> MSLRPCFVSLIDESDKPILIYVPNEAENEMNDVLKYNVLSNISLDYFESALVEWHSLDSKPLLKSIFQLEGVSVFAMLIKQTGLKIVIGFEQKSLSGADDEFEAINQIFETVRKIYIRVKCNPLLVSGDEKSIIKSLERKFDELFISTEVEL;> MSSTHSNNVGHPQSSPQGPLTEQQRAQQQYQIFENSLPKVSQSVYQMLLNEMVPLAMGIERQISGDVISSDSNVTSENGNINNMIKRLKIEEHHTVDIIRSHNLIHELYKADEEEKEKVLARLRNIGFQIGLKLSELLIFSNNPNLKFKEMDLLLIMKFICRDVWKQIFGKQIDNLKTNHRGTFYLLDYDYRPIQSFSLEEDAKNEELKMIEPFLEIPVGIIRGVLSSLGYSSEEVICLASFIDRPTDRPKTAFPKGVSFHVQVTMPQ;>[2x]MVSTTQSRSLKAMGEEIWKNKTEKINTELFTLTYGSIVAQLCQDYERDFNKVNDHLYSMGYNIGCRLIEDFLARTALPRCENLVKTSEVLSKCAFKIFLNITPNITNWSHNKDTFSLILDENPLADFVELPMDAMKSLWYSNILCGVLKGSLEMVQLDCDVWFVSDILRGDSQTEIKVKLNRILKDEIPIG;> MGIYSFWIFDRHCNCIFDREWTLASNSASGTINSKQNEEDAKLLYGMIFSLRSITQKLSKGSVKNDIRSISTGKYRVHTYCTASGLWFVLLSDFKQQSYTQVLQYIYSHIYVKYVSNNLLSPYDFAENENEMRGQGTRKITNRNFISVLESFLAPMVNQ;> MAIETILVINKSGGLIYQRNFTNDEQKLNSNEYLILASTLHGVFAIASQLTPKALQLTQQTNIENTIPYIPYVGMSSNRSDTRNGGGNNNKHTNNEKLGSFKGDDFFKEPFTNWNKSGLRQLCTDQFTMFIYQTLTGLKFVAISSSVMPQRQPTIATTDKPDRPKSTSNLAIQIADNFLRKVYCLYSDYVMKDPSYSMEMPIRSNLFDEKVKKMVENLQ;> MSQRIIQPSASDQQFPGKSDGYEYTVGPKQAITSEASTTYIPSRIYSESLLFKRQEASLSAMAFLFQEMISQLHRTCKTAGDFETKLSDYGHNIGIRLLELLNFRASVSPSSLPRASAFLSQNESSSKLSNASNSPGMLANSSTATSASANERLQEKQTESLSNYITKMRRRDLKILDILQFIHGTLWSYLFNHVSDDLVKSSERDNEYMIVDNFPTLTQFIPGENVSCEYFVCGIIKGFLFNAGFPCGVTAHRMPQGGHSQRTVYLIQFDRQVLDREGLRFG;> MPQYFAIIGKKDNPVYEIEFTNAENPQGFPQDLKELNPFILHASLDIVEDLQWQINPTSQLNGNGGNGSNGGGGFLRSRAVNNTDNCYLGKVDHFYGLAITAYISYSGMKFVMIHGNSANSSVVIDDNNMRSFYQEVHELYVKTLMNPFYKITDPIRSPAFDSRVRTLARKHLSK;> MDKEIYCGSVPVSYFDPFDLFESLRPEFQQILPLDNIHWKAFDGTVRTVNRLPIELIPEGRGEADKSNDEQPFIRFLIVNCISIDQYRAKVRPLVRQWLPNLESVSSSTGEKMIYKPIILLYANSEVVDSNLFKSVSLMEKFGKDFPHVQTLEVRSVYRSPKERQEFWNQFSQKIKASVLSIFQKRLTHLQHSLANLQKGNNFEEQLLTREKLYELYVVFNILEDASLELQKIKKEILRRNMNMPDGKLQVPFESSSKSDESLGSIIIEGTLDKFQLHKYFFIRRLRLLKLEDQTLTAFVGAFQLIKNFIESISIEYRKSVRLLEFKHYFITSMLSYFEFENVSNPLLCEIKAELLMLKRDNWVQGVMATSGYRLMDKNYPNSDVKYKFDLLKETFVDETVFQENFLTLTKEILSLFNKCEGKRQRIVDILSIEIGLLYYQGKKYEEAVSLFLSCYEYYTQTNWNSIGLKILQVFIDSLSHCPKLDVLQIDGESVSASAVLTNAFLNILKLCKDNDSKEIWWKKFMDLQMKNNIHLMYPLDGLFEVTLNSKVHLARANVSAIEVNLKSYGFPEDISTKTMRLSLKNMGGDVIVFGASDFLLKKGENKLILECRDIMYGEFSLLSFEIIVEGITFVKEFPENQDEFIVVPEIYCKESTKVLVKQAHNLNLGEYALELKSVQSDALESLQVEVEVQKNIGNMKNLPVSFSMDEIQARKRYNTPFENVRLEYYLLDQITAFDLIIKTSFTKKNDQGTFGETKKVRIQCYLQLSVSVEDIFKKDIFFFKFLLNSSVREEPVILYSSELSAPDTRNDYNIRGDYIATTPALITFDGNESFINCYEITANNNFDSKDIFNLKVRYNTLKEQLDCFITDAVLIEGDVEWFILFEKWKTFWELEILKKLKYDYDAFKENRIIRLLKTSIDLNKTKSKIRNLCIEKAVLDKILICLNKVSRGIAVCNTDMDEYVRNLVPKQLTVPVQLPGFEQFFHVQFEQMETSHDALHDTIATIGNSLSYTVIVENLSGQWGQDVIDDGGYIFEILSSNEWLIHGQKRCAIKEKRKEFEVHLIPLKKGYLNFPRVEITNINGKSCRVDHSNAFESILIF;> MNILKHFPSYVGPSKIRTLVIPIGHWTRKEFNNAVQKLSEFNEIHLSDVTPIDSPIFTPQGFPHGKLFFDFLTIDHDDALELFLYDFEPFRKTFVIIGLVNDYSDPLTNLNFMKEKYPTLISPNLVYASSTPTKELEQTIDTMENVFASSPDMQKNIETIMCDIARNFLTALNSYYSSYKHVTLRSPGAIGGNAVLKTTLIRQNSYTSSSSSTPMSAVQSSVSSSSKAGSVTTASKRLSSFEMTTNSLKRSASLKLATTLSTSENRSQQKSLGRQMKILGNFQLLAGRYVDALNSFVDAITTLYKVRDYLWLGSALDGISICFLLLSYLGLSYQIPQIVSLICPVEKLNFESSSTGISPVDSNSKATASTTASSTPRNSISIAAMQSPRNSIMSLSAPALNIDVENINLPLLIKCISDKVLYYYDLSLMHNSEYAPQVVYCEFLLKTLTFMTSCYKSSEFSKDVLDNIVKNQHRALSDIPNSPMFPRFEVYFYSNKLFELQLKEMQVEAQIKIYSTMAEVYRLLGYKRKQLFVLRLLMVALLATPNKIAWHPDYRTLIDTIIELLNINESEAKINVDDPSQSTWLILQKKILQLCIKVSRKINDFEYVAKFSSILITKYTHLLNQSEQDALFKEYIQPSITNESITSYWDPFILREVVINRILDSDPTSNEIPLESDVSSLESLENRQKTQDINPQEVFNPFKRVQPTSFVSNNSTKVPILVFLVGDKAEFTCRVQNPFKFDFTINDIQLDEEISEFCEIDRKAVSYSGPYNVKAESIRSITLPLIIKKPTYKKIYEISCLKISILKLPLQKFDIINDSRRSNPVEEEAEYSKCIYGKLKIKILPEQPQLELLSTSKMTRNSWMMLDGTKTDFHITVRNKSLSCAINHIKIIPMNNIEQMLKPDYWKKMPPDDLYIMEKQLDWLSKSCVRIIKLPTVIKPNETITFDLELDNTAVPFNFTGFDLLIEYGMSATDESCIYLKKLSIPYEVTLRRTIEVPSMDIIPLNELFSSQVENVDWIEYVMSKIRAESNLHSRDFILLLLDFRNSWIDGIKLNVQFEDFTSNE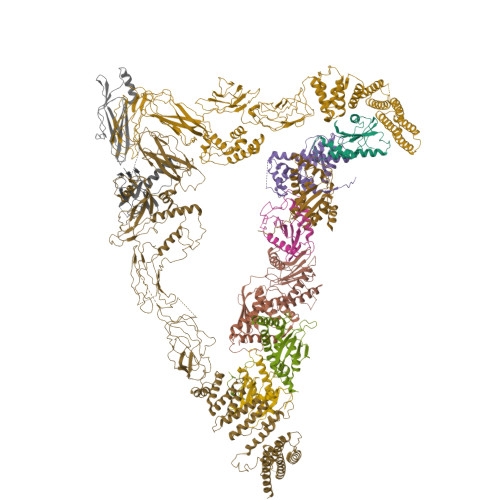YHVEASHTSRIIVPIKKIDYKKYNFENTPIPRIYPGRQFIQSGLNEEQTIEMRQKFWCREHIISKLKCNWKLTTDQSVTGSVDFNKFIEKFDHKMVYTIYPGRLFYGVQLLLDEPKVKVGEIINLKIITEPTSTCRRKQNSTVNFLDIVIFDSKTSKILPRSNRRILYNGSLTKPISTTKVSEINLEIIPIEKGRYEFSVCISKSNNQDGIIQFDSENVILSVI;> MECFVPLRCDLDGSNIEQLRQSHLSRKFIIFDEQLNLWLWFQGNSQENKRFVLQNMIILINEAQVTRTSTIDDYFTQVENNENLWRLKNDCCSKILFKSNVVMNNGYNNQIKFVFEYKSVDANFNNQDSLQDPQAKYTLDKYSSEEILPSFEPVYSWSSAATKSSKNTNNHLEKNNRATHRVSSKNSEVHEADVSRNPNTFTLKLQYPIFSLLNMRLRNISLKSEHCILSSLDFQTSKASEQLTKKFIYPQEHNSFLKLNFQEISYKLIDGTSQIELDPICPLKVPLTAFSYDSISATFKLVLLPKSTQPHRVKITLAYELELHPNLKLPVRTSWETEVTLKRSMPISSTSSQYSSNNNNTNHSASFNGAANNVNSGGLANLRLGGVSSSRFSLGAASTTSLVNSKLSNVKFKFINSNIKVIKGEKFTMRLQIINSSSSPLDLVVYYNNTINPIPSANNVRNSNGINNCGMNNGTIPNSPLTLENQYQLHNKYRKIAEGIILLSNDYKIPVVPPRETYFADLRFIGIMSGYYGTLSGLKVLDLNTNELIEVGNGASVLIQ>[2x]IAPLVGYAIGAAAISAVGGIGVGWTLREFEVVGSDDPAEGLTPDVLRNQLSDSVVKRKSNNQSTMVDNQNILDGVEHTAYTEAKIAAIEELNAGSSESAVLSAANSAIDSYETTVRTNFYKSWNETVRELEAMTQTVIAHADVGLSYITDFGDPRFGNLASGTSPNTLKDTTVSMPDGTNFTLLTFRHNTGWDSGNAAYSVVEYNPKEVVTSTNSNTYNTVDGTQYMKFSEWNAVETEMDTVFQNVRNGISTWVTNVYGDVQSGAIEISDLVTPRERATMMAQEEGMSQAIADLIALNVPVDAEREATITIQDTGATLPGTFALTDSSDGPLSAGQTYDPSTFSGDVYFTADMSLVEGPWDAINSGVDGGTITITSEPYEGTAIEVTTVESETVSVPAADWTDN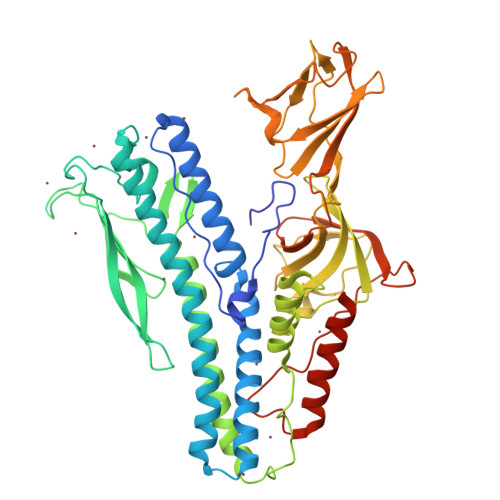GDGTWSYDASGDLETTITNVDSARFVSTATETTYDTLQLKGAFTVDKLVNKQSGEEVSSTSFTSSEPQTDSNYITQDEWDQLEQQNKELIEKYEQSQSGGGLDLGGLD> HHHHHHGPEHEFVRALIKRNCHVITTSKGEFNMLGIHDNCAVVPTHAECGDSVTIDGREVRVLKQCILTDTNDTDTEITLLWLDQNEKFRDIRRFIPEHQREWSNMHLATNVTKFPMLDVEVGTVIPYGEVNLSGNPTCRLLKYNYPTKPGQ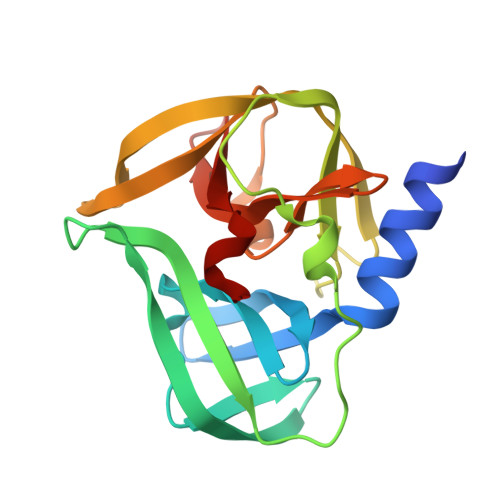CGGVIANTGNIVAIHVGGNGRVGYGAALLRKYFA>YKKAGLQRTLVLIKPDAFERSLVAEIMGRIEKKNFKIVSMKFWSKAPRNLIEQHYKEHSEQSYFNDLCDFMVSGPIISIVYEGTDAISKIRRLQGNILTPGTIRGDL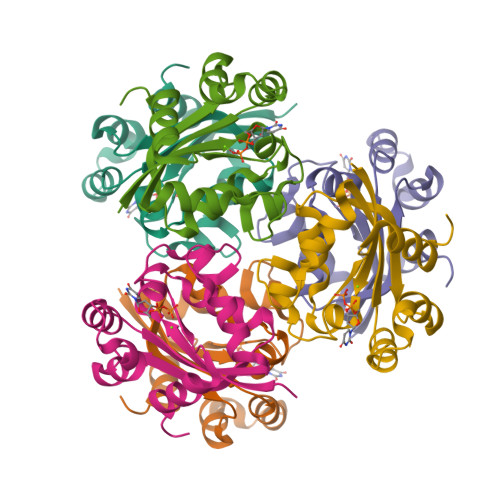ANDIGENLIHASDSEDSAVDEISIWFPETKMETDN[6x]> GPLCAQEFSDLTDPLYIKKICLEKVPEWNHFTEDNLRVKQILSGLTNQLFEVGLKEETANNYNSIRTRVLFRIYGKHVDELYNTISEFEVYKTMSKYKIAPQLLNTFNGGRIEEWLYGDPLRIDDLKNPTILIGIANVLGKFHTLSRKRHLPEHWDRTPCIFKMMEKWKNQLFKYKNIEKYNCDIHKYIKESDKFIKFMKVYSKSDNLANTIVFCHNDLQENNIINTNKCLRLIDFEYSGFNFLATDIANFFIETSID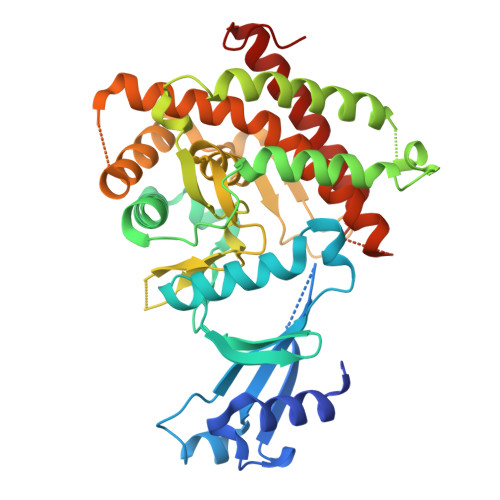YSVSSYPFFEIDKKKYISYENRKLFITAYLSNYLDKSLVVPTPKLIDEILEAVEVQALGAHLLWGFWSIIRGYQTKSYNEFDFFLYAEQRLKMYDDQKEYLISNNIIKGYD> HHHHHHGLVPRGSHMTAQTVTGAVAAAQLGATLPHEHVIFGYPGYAGDVTLGPFDHAAALASCTETARALLARGIQTVVDATPNGCGRNPAFLREVSEATGLQILCATGFYYEGGGATTYFKFRASLGDAESEIYEMMRTEVTEGIAGTGIRAGVIKLASSRDAITPYEQLFFRAAARVQRETGVPIITHTQEGQQGPQQAELLTSLGADPARIMIGHMDGNTDPAYHRETLRHGVSIAFDRIGLQGLVGTPTDAERLSVLTTLLGEGYADRLLLSHDSIWHWLGRPPAIPEAALPAVKDWHPLHISDDILPDLRRRGITEEQVGQMT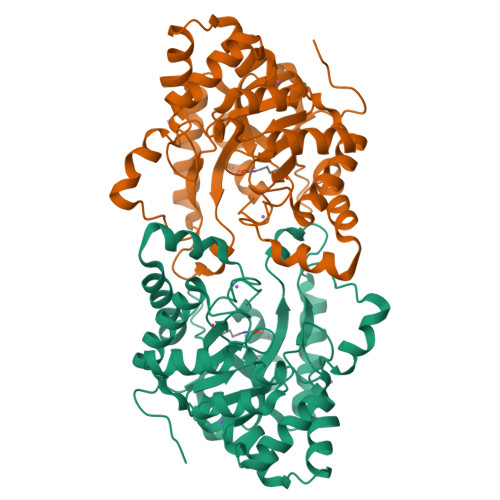VGNPARLFG> MGSSHHHHHHSQDPTVPAQLQFSAKTLDGHDFHGESLLGKPAVLWFWAPWCPTCQGEAPVVGQVAASHPEVTFVGVAGLDQVPAMQEFVNKYPVKTFTQLADTDGSVWANFGVTQQPAYAFVDPHGNV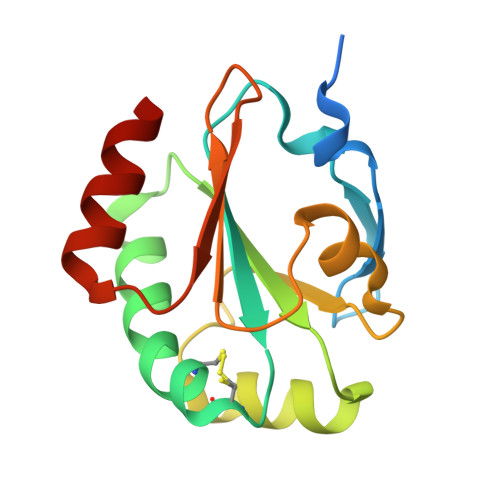DVVRGRMSQDELTRRVTALTSR> SHLKSKKGQ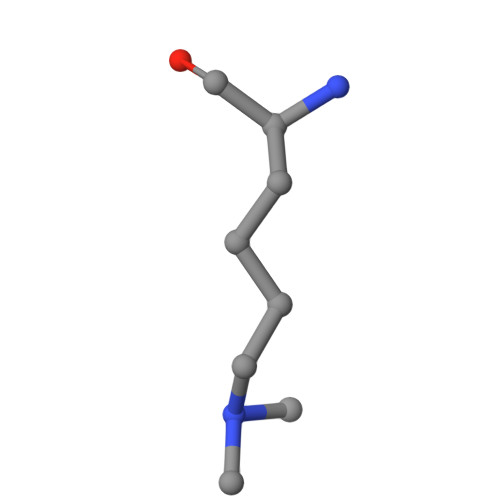ST2'-deoxy-2'-(2-hydroxyethyl)adenosine 5'-(trihydrogen diphosphate) | C12 H19 N5 O10 P2 | 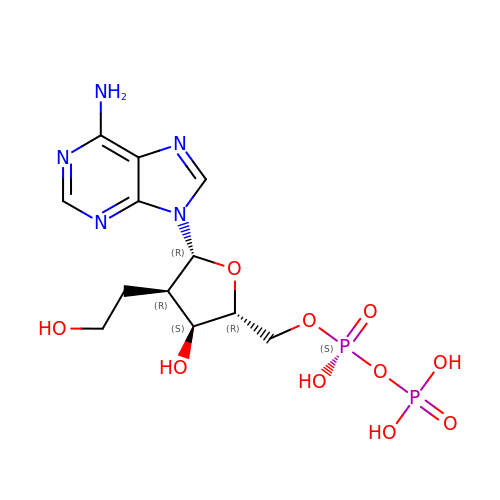RHTGRZKDKXTTPI-PNFUHCLESA-N> SNQTFTYINYYKDAASTSSAGQSLSMDPSKFTEPVKDLMLKGA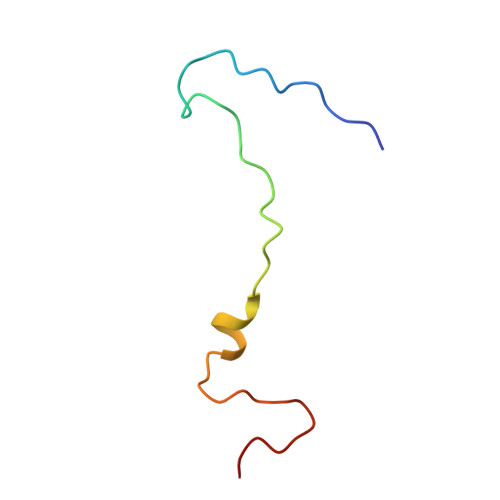PALN>GSHMRRRVRAILPYTKVPDTDEISFLKGDMFIVHNELEDGWMWVTNLRTDEQGL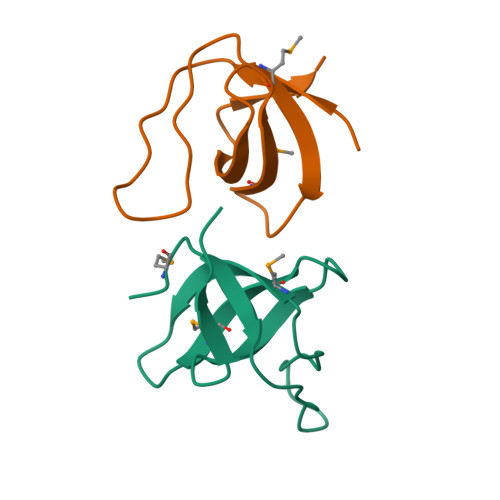IVEDLVEEVGR[2x]> TYMNN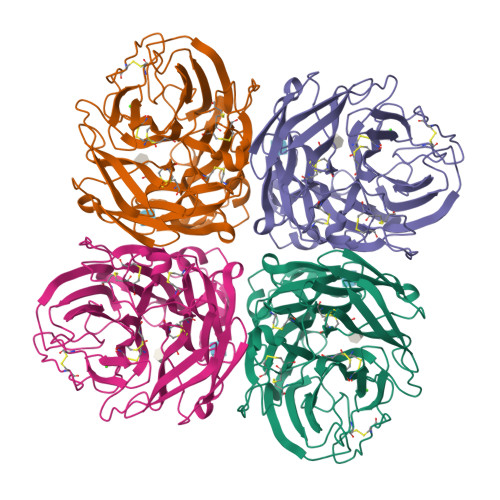TEAICDAKGFAPFSKDNGIRIGSRGHIFVIREPFVSCSPIECRTFFLTQGSLLNDKHSNGTVKDRSPFRTLMSVEVGQSPNVYQARFEAVAWSATACHDGKKWMTVGVTGPDSKAVAVIHYGGVPTDVVNSWAGDILRTQESSCTCIQGDCYWVMTDGPANRQAQYRIYKANQGRIIGQTDISFNGGHIEECSCYPNDGKVECVCRDNWTGTNRPVLVISPDLSYRVGYLCAGIPSDTPRGEDTQFTGSCTSPMGNQGYGVKGFGFRQGTDVWMGRTISRTSRSGFEILRIKNGWTQTSKEQIRKQVVVDNLNWSGYSGSFTLPVELSGKDCLVPCFWVEMIRGKPEEKTIWTSSSSIVMCGVDYEVADWSWHDGAILPFDI> MDKYTALIHDENFSTLTLNVSRYPKSLAYWEKLLNYIVKASAPICKSTEPQLLKLIRCTYSSMLNEFPYLENYYIDFALLEYKLGNV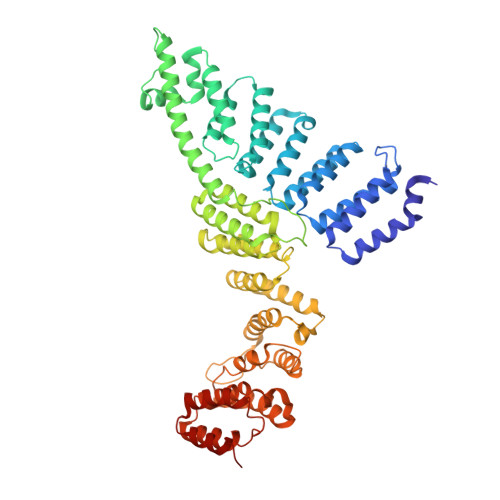SMSHKIFQRGLQAFNQRSLLLWTSYLKFCNNVISHQKQLFKKYETAEEYVGLHFFSGEFWDLYLEQISSRCTSSKKYWNVLRKILEIPLHSFSKFYALWLQRIDDIMDLKQLSQLTSKDELLKKLKIDINYSGRKGPYLQDAKKKLKKITKEMYMVVQYQVLEIYSIFESKIYINYYTSPETLVSSDEIETWIKYLDYTITLQTDSLTHLNFQRALLPLAHYDLVWIKYSKWLINSKNDLLGAKNVLLMGLKFSLKKTEIIKLLYSVICKLNEYVLLRNLLEKIESSYSDNVENVDDFEIFWDYLQFKTFCQNSLYSSRYSDSQSNGLLNKELFDKVWKRLSCKEKKSGQEILLNNLVQFYSKDTVEFVEKNIFQKIIEFGWEYYLQNGMFWNCYCRLIYFDTSRSYLDKRQYIVRKIWPQIDKKFAQSVLPSLTEFCESYFPEEMDTLEEMFTEEP>TTSSSDGIPKSEASERIKTGFLHFKKEKYDKNPALYGELAKGQSPPFMVFACSDSRVCPSHVLDFQPGEAFVVRNVANLVPPYDQAKYAGTGAAIEYAVLHLKVSNIVVIGHSACGGIKGLLSFPFDGTYSTDFIEEWVKIG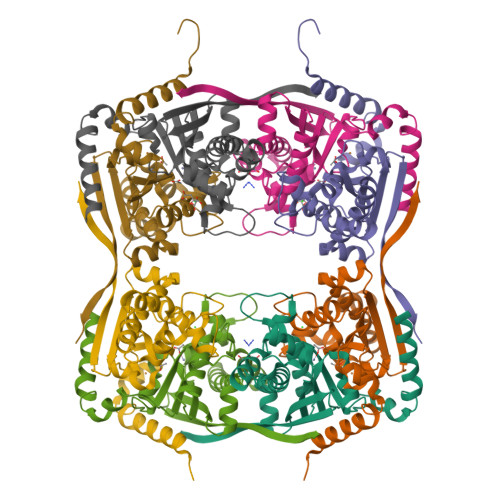LPAKAKVKAQHGDAPFAELCTHCEKEAVNASLGNLLTYPFVREGLVNKTLALKGGYYDFVKGSFELWGLEFGLSSTFSV[8x]>[6x]MTSAEMTSPNNNSEHQAIAKMRTMIEGFDDISHGGLPIGRSTLVSGTTGTGKTLFSIQFLYNGIIEFDEPGVFVTFEETPQDIIKNARSFGWDLAKLVDEGKLFILDASPDPEGQEVVGGFDLSALIE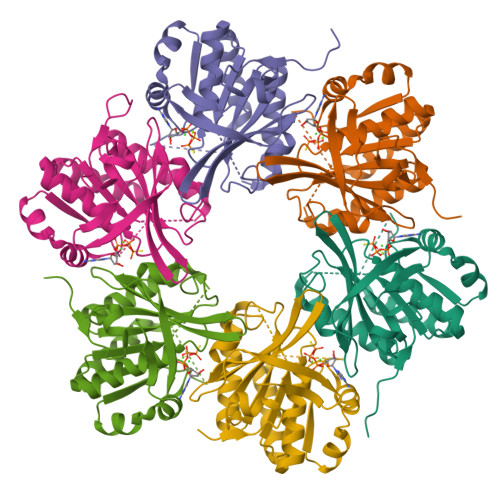RINYAIQKYRARRVSIDSVTSVFQQYDASSVVRRELFRLVARLKQIGATTVMTTERIEEYGPIARYGVEEFVSDNVVILRNVLEGERRRRTLEILKLRGTSHMKGEYPFTITDHGINIFPLGAMR> SQIPASEQETLVRPKPLLLKLLKSVGAQKDTYTMKEVLFYLGQYIMTKRLYDEKQQHIVYCSNDLLGD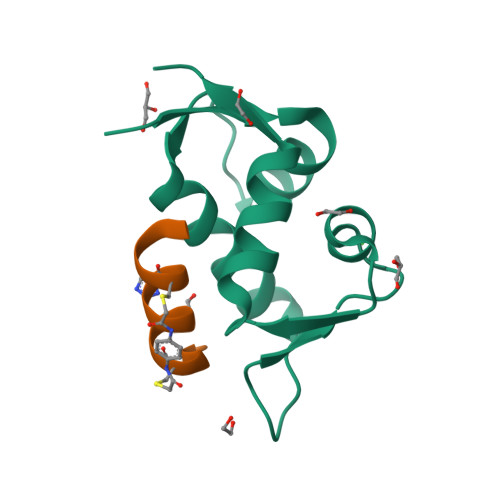LFGVPSFSVKEHRKIYTMIYRNLVVVN;> XDPAWNHCEYAAFVCSEVX> SGISLDNSYKMDYPEMGLCIIINNKNFHKSTGMTSRSGTDVDAANLRETFRNLKYEVRNKNDLTREEIVELMRDVSKEDHSKRSSFVCVLLSHGEEGIIFGTNGPVDLKKITNFFRGDRCRSLTGKPKLFIIQACRGTELDCGIETD;> SGVDDDMACHKIPVDADFLYAYSTAPGYYSWRNSK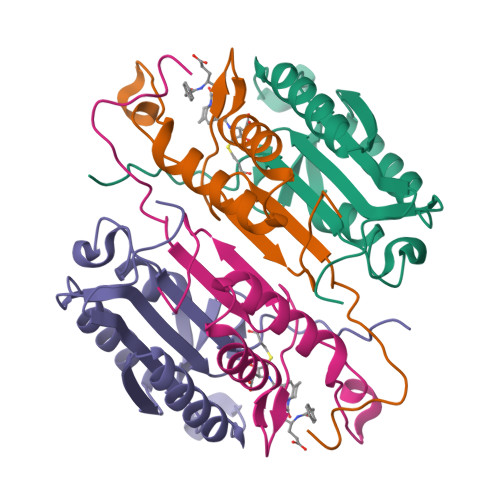DGSWFIQSLCAMLKQYADKLEFMHILTRVNRKVATEFESFSFDATFHAKKQIPCIVSMLTKELYFYHHHHHHHH> LEEDGTIITL;> GPGSEFGTREFLTFEVPLNDSGSAGLGVSVKGNRSKE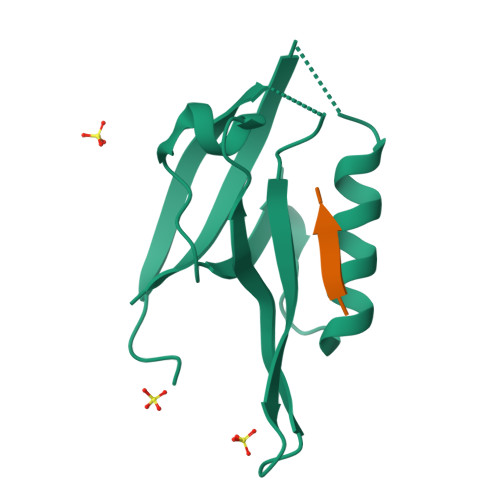NHADLGIFVKSIINGGAASKDGRLRVNDQLIAVNGESLLGKANQEAMETLRRSMSTEGNKRGMIQLIVARRIS(3~{R})-1-[(2~{R})-2-[4-(2-chloranyl-4-fluoranyl-phenyl)-2-oxidanylidene-chromen-7-yl]oxypropanoyl]piperidine-3-carboxylic acid | C24 H21 Cl F N O6 | 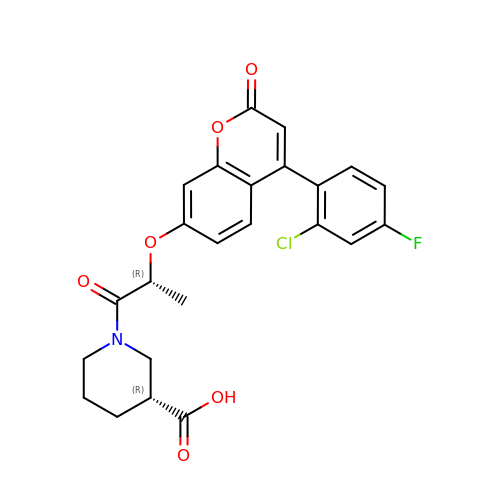PFEKWBKJUBCXDT-ZIAGYGMSSA-N>ADKLFINALKKKFEESPEEKKTTFYTLGGWKQSERKTEFVNAGKEVAAKRGIPQYNPDIGTPLGQRVLMPYQVSTTDTYVEGDDLHFVNNAAMQQMWDDIRRTVIVGLNHAHAVIEKRLGKEVTPETITHYLETVNHAMPGAAVVQEHMVETHPALVADSYVKVFTGNDEIADEID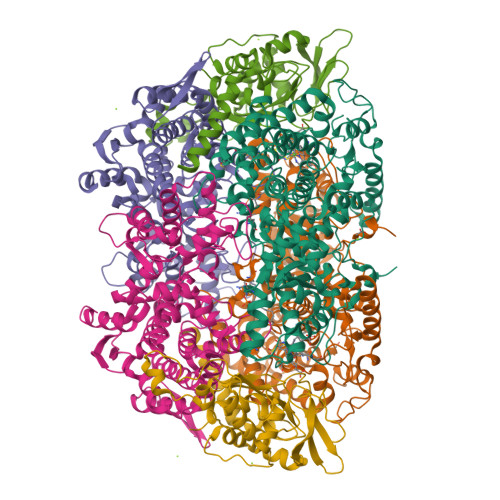PAFVIDINKQFPEDQAETLKAEVGDGIWQVVRIPTIVSRTCDGATTSRWSAMQIGMSMISAYKQAAGEAATGDFAYAAKHAEVIHMGTYLPVRRARGENEPGGVPFGYLADICQSSRVNYEDPVRVSLDVVATGAMLYDQIWLGSYMSGGVGFTQYATAAYTDNILDDFTYFGKEYVEDKYGLCEAPNNMDTVLDVATEVTFYGLEQYEEYPALLEDQFGGSQRAAVVAAAAGCSTAFATGNAQTGLSGWYLSMYLHKEQHSRLGFYGYDLQDQCGASNVFSIRGDEGLPLELRGPNYPNYAMNVGHQGEYAGISQAPHAARGDAFVFNPLVKIAFADDNLVFDFTNVRGEFAKGALREFEPAGERALITPA[2x];>[2x]AKFEDKVDLYDDRGNLVEEQVPLEALSPLRNPAIKSIVQGIKRTVAVNLEGIENALKTAKVGGPACKIMGRELDLDIVGNAESIAAAAKEMIQVTEDDDTNVELLGGGKRALVQVPSARFDVAAEYSAAPLVTATAFVQAIINEFDVSMYDANMVKAAVLGRYPQSVEYMGANIATMLDIPQKLEGPGYALRNIMVNHVVAATLKNTLQAAALSTILEQTAMFEMGDAVGAFERMHLLGLAYQGMNADNLVFDLVKANGKEGTVGSVIADLVERALEDGVIKVEKELTDYKVYGTDDLAMWNAYAAAGLMAATMVNQGAARAAQGVSSTLLYYNDLIEFETGLPSVDFGKVEGTAVGFSFFSHSIYGGGGPGIFNGNHIVTRHSKGFAIPCVAAAMALDAGTQMFSPEATSGLIKEVFSQVDEFREPLKYVVEAAAEIKNEI;>[2x]AQYYPGTTKVAQNRRNFCNPEYELEKLREISDEDVVKILGHRAPGEEYPSVHPPLEEMDEPEDAIREMVEPIDGAKAGDRVRYIQFTDSMYFAPAQPYVRSRAYLCRYRGADAGTLSGRQIIETRERDLEKISKELLETEFFDPARSGVRGKSVHGHSLRLDEDGMMFDMLRRQIYNKDTGRVEMVKNQIGDELDEPVDLGEPLDEETLMEKTTIYRVDGEAYRDDVEAVEIMQRIHVLRSQGGFN>[6x]HDTTVFQGVAGQSLQVSCPYDSMKHWGRRKAWCRQLGEKGPCQRVVSTHNLWLLSFLRRWNGSTAITDDTLGGTLTITLRNLQPHDAGLY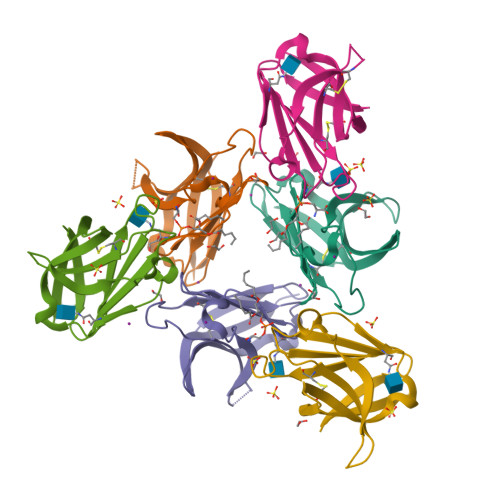QCQSLHGSEADTLRKVLVEVLADPLDHRDAGDLWFPGESESFEDAHVEHSISRSLLEGEIPFPPTSENLYFQGHHHHHH>[2x]MKKGHHHHHHENLYFQGGSLKLSAENESTPIQQLLEHFLRQL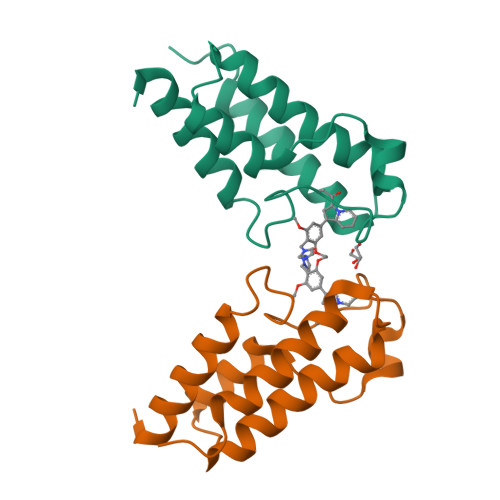QRKDPHGFFAFPVTDAIAPGYSMIIKHPMDFGTMKDKIVANEYKSVTEFKADFKLMCDNAMTYNRPDTVYYKLAKKILHAGFKMMSKERLLALKRSMSFMQDMDFSQ>MHHHHHHHHHHENLYFQGGSMAQVINTNSLSLLTQNNLNKSQSALGTAIERLSSGLRINSAKDDAAGQAIANRFTANIKGLTQASRNANDGISIAQTTEGALNEINNNLQRVRELAVQSANSTNSQSDLDSIQAEITQRLNEIDRVSGQTQFNGVKVLAQDNTLTIQVGANDGETIDIDLKQINSQTLGLDTLNVQQKYKVSDTAATVTGYADTTIALDNSTFKASATGLGGTDQKIDGDLKFDDTTGKYYAKVTVTGGTGKDGYYEVSVDKTNGEVTLAGGATSPLTGGLPATATEDVKNVQVANADLTEAKAALTAAGVTGTASVVKMSYTDNNGKTIDGGLAVKVGDDYYSATQNKDGSISINTTKYTADDGTSKTALNKLGGADGKTEVVSIGGKTYAASKAEGHNFKAQPDLAEAAATTTENPLQKIDAALAQVDTLRSDLGAVQNRFNSAITNLGNTVNNLTSARSRIEDSDYATEVSNMSRAQILQQAGTSVLAQANQVPQNVLSLLRGSGAGGSEGGMASISSLGVGSNLPLDQLLTDLTKNEKGRLTPITKQQSANSAKLTAYGTLKSALEKFQTANTALNKADLFKSTVASSTTEDLKVSTTAGACAGTYKINVTQLAAAQSLATKTTFATTKEQLGDTSVTSRTIKIEQPGRKEPLEIKLDKGDTSMEAIRDAINDADSGICASIVKVKENEFQLVLTANSGTDNTMKITVEGDTKLNDLLAYDSTTNTGNMQELVKAENAKLNVNGIDIERQSNTVTDAPQGITLTLTKKVT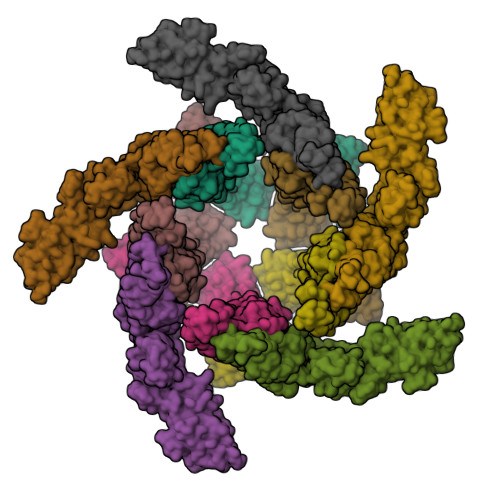DATVTVTKDDTKAKEAIKSWVDAYNSLVDTFSSLTKYTAVEPGEEASDKNGALLGDSVVRTIQTGIRAQFANSGSNSAFKTMAEIGITQDGTSGKLKIDDDKLTKVLKDNTAAARELLVGDGKETGITTKIATEVKSYLADDGIIDNAQDNVNATLKSLTKQYLSVSNSIDETVARYKAQFTQLDTMMSKLNNTSSYLTQQFTAMNKS[10x]To initiate filament growth, three junction proteins, namely, FlgK (hook-associated protein 1), FlgL (hook-associated protein 3), and the cap protein FliD (hook-associated protein 2), are sequentially placed at the distal end of the hook. The FlgL and FlgK junction proteins that are located between the FlgE hook and the flagellin filament are indispensable for the formation of the flagellum because both FlgL-deficient bacteria and FlgK-deficient bacteria lack functional flagella and are immotile. To investigate the role of FlgL in hook-filament assembly, we have determined the crystal structures of FlgL from gram-positive Bacillus cereus (bcFlgL) and gram-negative Xanthomonas campestris (xcFlgL). The bcFlgL and xcFlgL structures revealed that the D1 domain of FlgL forms a four-segment structure, irrespective of the bacterial species.

Crystal structures for the truncated bcFlgL and xcFlgL proteins (residues 45–251 and residues 48–364, respectively), which lack ~45 N-terminal residues and ~35 C-terminal residues, were solved by multiwavelength anomalous diffraction (MAD) phasing and single-wavelength anomalous diffraction (SAD) phasing, respectively. The bcFlgL structure was refined to 2.2 Å resolution. xcFlgL was crystallized in two different crystal forms, and we obtained two xcFlgL structures (xcFlgLC2 structure in space group C2 at 1.9 Å resolution; xcFlgLH3 structure in space group H3 at 2.2 Å resolution; xcFlgL structure refers to xcFlgLC2 unless specified). The truncated bcFlgL and xcFlgL proteins adopt one-domain (D1) and two-domain (D1-D2) structures, respectively. xcFlgL contains an additional domain, D2, compared to bcFlgL. The D2 domain of xcFlgL forms a β-sandwich structure, which consists of a β5-β12-β7-β8-β9 sheet and a β6-β11-β10 sheet. Notably, the D1-D2 interdomain orientation and interface are essentially identical in the two crystal structures of xcFlgL (xcFlgLC2 and xcFlgLH3) despite different crystal contacts, suggesting that the D1-D2 orientation would not change in different environments and would be recapitulated both in solution and in the flagellum. Our comparative analysis of the two xcFlgL structures (xcFlgLC2 and xcFlgLH3) indicates that the N-terminal and C-terminal regions of the FlgL D1 domain adopt diverse conformations, as observed for flagellin. In the xcFlgLC2 structure, the α4b helix runs downwards as one α-helix. However, in the xcFlgLH3 structure, the α4b helix is split into two discontinuous α-helices (α4b and α4c) due to a sharp directional change in the helix. Moreover, the N-terminal regions of the α1 helices are tilted in different directions in the two xcFlgL structures.

>[2x]GSAKDPAGTAVGLDRALAAITRFGENANNVQNRLGLQENALAQAGDKMARVTELAVQSNNSSLSPDDRKAIASELTALRDSMVSLANSTDGTGRYLFAGTSDGNAPFIKSNGNVLYNGDQTQKQVEVAPDTFVSDTLPGSEIFMRIRTGDGSVDAHANATNTGTGLLLDFSRDASSGSWNGGSYSVQFTAADTYEVRDSTNALVSTGTYKDGEDINAAGVRMRISGAPAVGDSFQIGASGTKDVFSTIDDMVAALNSDTQTPTQKAAMINTLQSSMRDIAQASSKMIDARASGGAQLSVIDNANSLLESNEVTLKTTLSSIRD> YDNPIFEKF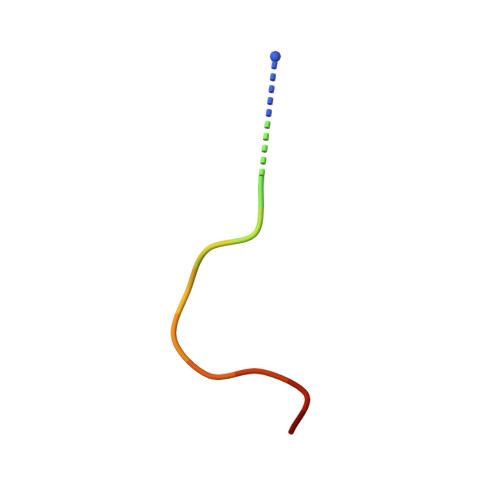GKGGTYX>[5x]DYKDDDDKMVVVTGREPDSRHSDGAMSSSEAEDDFLEPATPTATQAGHGLPLLPQEFPEVVPLNIGGAHFTTRLSTLRRYEDTMLAAMFSGRHYIPTDSEGRYFIDRDGTHFGDVLNFLRSGDLPPREHVRAV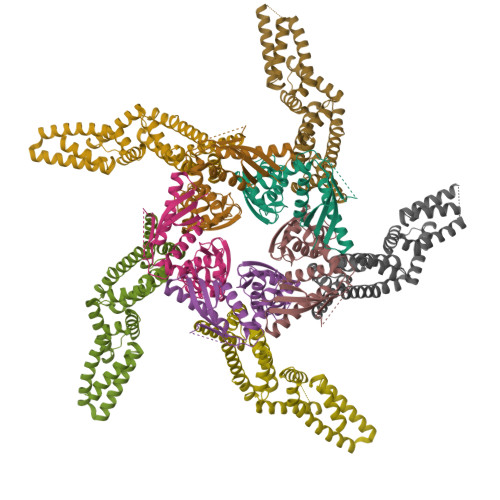YKEAQYYAIGPLLEQLENMQPLKGEKVRQAFLGLMPYYKDHLERIVEIARLRAVQRKARFAKLKVCVFKEEMPITPYECPLLNSLRFERSESDGQLFEHHCEVDVSFGPWEAVADVYDLLHCLVTDLSAQGLTVDHQCIGVCDKHLVNHYYCKRPIYEFKITWW;>[5x]MHHHHHHGSPMTMDEKYVNSIWDLLKNAIQEIQRKNNSGLSFEELYRNAYTMVLHKHGEKLYTGLREVVTEHLINKVREDVLNSLNNNFLQTLNQAWNDHQTAMVMIRDILMYMDRVYVQQNNVENVYNLGLIIFRDQVVRYGCIRDHLRQTLLDMIARERKGEVVDRGAIRNACQMLMILGLEGRSVYEEDFEAPFLEMSAEFFQMESQKFLAENSASVYIKKVEARINEEIERVMHCLDKSTEEPIVKVVERELISKHMKTIVEMENSGLVHMLKNGKTEDLGCMYKLFSRVPNGLKTMCECMSSYLREQGKALVSEEGEGKNPVDYRQGLDDLKSRFDRFLLESFNNDRLFKQTIAGDFEYFLNLNSRSPEYL>PPYTVVYFPVRGRCAALRMLLADQGQSWKEEVVTVETWQEGSLKASCLYGQLPKFQDGDLTLYQSNTILRHLGRTLGLYGKDQQEAALVDMVNDGVEDLRCKYISLIYTNYEAGKDDYVKALPGQLKPFETLLSQNQGGKTFIVGDQISFAAYNLLDLLLIHEVLAPGCLDAFPLLSAYVGR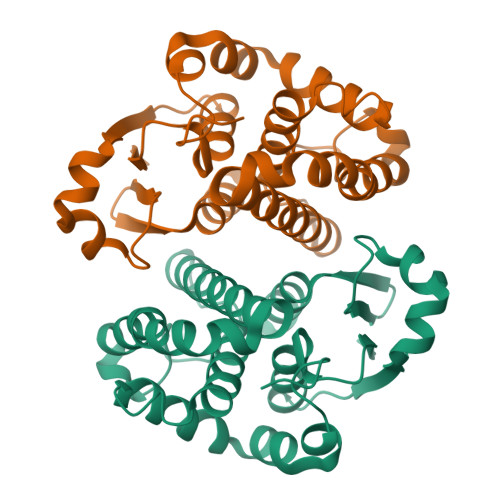LSARPKLKAFLASPEYVNLPINGNGKQ[8x]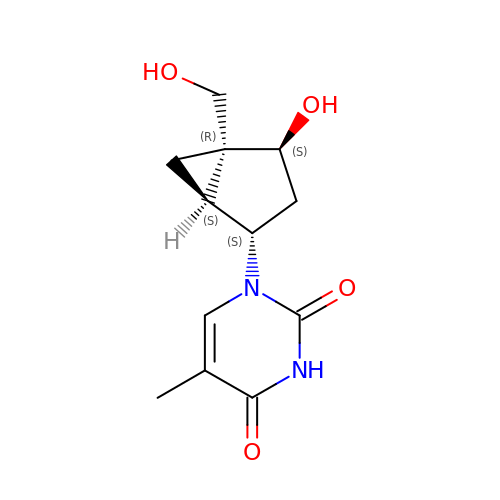1-[4-HYDROXY-5-(HYDROXYMETHYL)BICYCLO[3.1.0]HEX-2-YL]-5-METHYLPYRIMIDINE-2,4(1H,3H)-DIONE | C12 H16 N2 O4 | NOWRLNPOENZFHP-ARHDFHRDSA-N>[2x]MEQRVVIATTGGTYEKALREAWFEPFTKATGIKVVTVSGTDAEKRAKVTAMVQTGNVTWDLYLDGEIQAGSDAHFAITEDLSDFCMQFINSTDLLADSCTRGGAKLQSTSTLLAYKLNENGSNPQTWADMWDLAKFPGARSF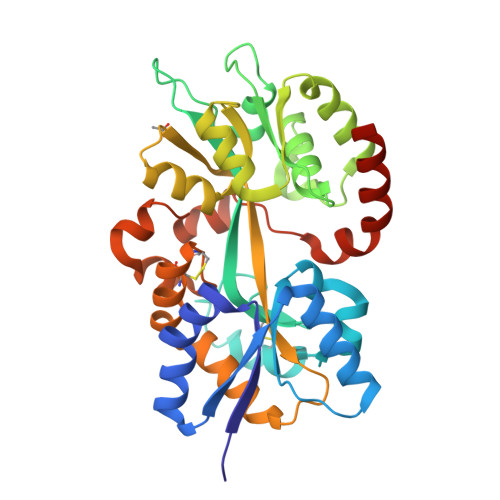PNFDDPWRVLAAALLADGVPREKLFPLDVDRAFRKLDELRDSVQVWWRTGDQSVQAFRNDEYRVGQIWLTRAKALKAEGYKIGWSYDGAFLVGDRIALVRGAPNRENALKLIEFWLRNPAAQAKACETLSCTPPSQKAISQMSSEARATLPSAADVENRIIVPDAQWINANMGMLVQRWNSWIRHHHHHH>[4x]MNIQNPVLKGFNPDPSIVRAGDDYYIATSTFEWFPGVQIHHSKDLVHWHLVAHPLSTTEFLDMKGNPDSGGIWAPDLSYADGKFWLIYTDVKVVDGMWKDCHNYLTTAEDIKGPWSKPILLNGAGFDASLFHDPSGKKYLVNMYWDQRVYHHNFYGIA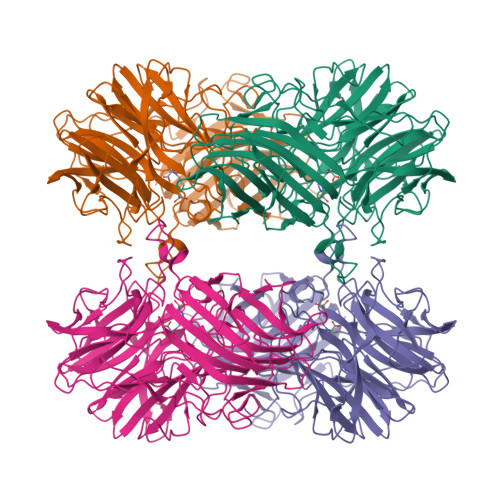LQEYSVAEEKLIGKPEIIYKGTDIAYTEGPHLYYINDMYYLMTAEGGTTYQHSETIARSKTIHGPYEIQPDYPLLSAWKEVHNPLQKCGHASLVETQNGQWYLAHLTGRPLPAPAGFPSREREQHAFCPLGRETAIQKIEWQDGWPVVVGGQQGSLEVEAPDLPQQEWAPTYEERDDFDKDTLNINFQTLRIPFSEHLGSLTARPGFLRLYGRESLQSKFTQAHIARRWQSFNFDAGTSVEFSPNSFQQMAGLTCYYNTENWSSIHVTWNEEKGRIIDLVTADNGTFSMPLAGAEIPIPDEVKTVHFKVSVRGRIYQYAYSFDGETFHTLPIELPSWKLSDDYVRGGGFFTGAFVGINAIDITGTALPADFDYFTYKELD5-(2-AMINOETHYL)-3-{5-[AMINO(IMINIO)METHYL]-1H-BENZIMIDAZOL-2-YL}-1,1'-BIPHENYL-2-OLATE | C22 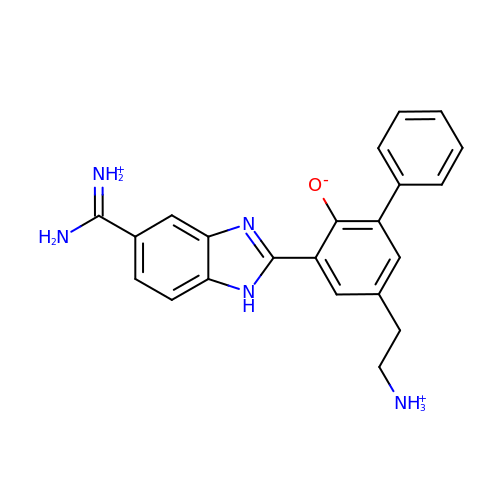H22 N5 O | YYUZFCLHOQHMPT-UHFFFAOYSA-O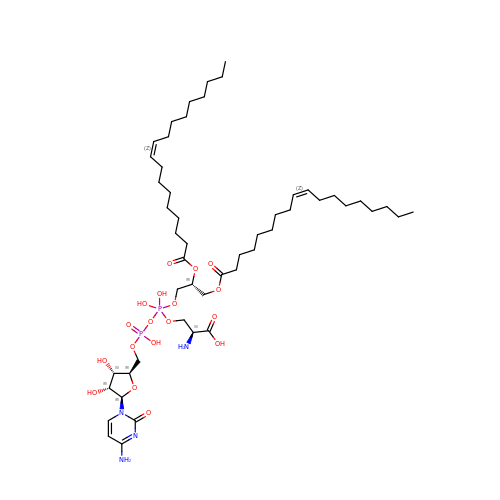(2S)-2-amino-3-[[[(2R,3S,4R,5R)-5-(4-amino-2-oxo-pyrimidin-1-yl)-3,4-dihydroxy-tetrahydrofuran-2-yl]methoxy-hydroxy-phosphoryl]oxy-[(2R)-2,3-bis[[(Z)-octadec-9-enoyl]oxy]propoxy]-dihydroxy-lambda^5-phosphanyl]oxy-propanoic acid | C51 H92 N4 O18 P2 | SMGJVPWANUHLFX-OTXLWCCGSA-N>[4x]MNAAAVTPPPEKFNFAEHLLQTNRVRPDKTAFVDDISSLSFAQLEAQTRQLAAALRAIGVKREERVLLLMLDGTDWPVAFLGAIYAGIVPVAVNTLLTADDYAYMLEHSRAQAVLVSGALHPVLKAALTKSDHEVQRVIVSRPAAPLEPGEVDFAEFVGAHAPLEKPAATQADDPAFWLYSSGSTGRPKGVVHTHANPYWTSELYGRNTLHLREDDVCFSAAKLFFAYGLGNALTFPMTVGATTLLMGERPTPDAVFKRWLGGVGGVKPTVFYGAPTGYAGMLAAPNLPSRDQVALRLASSAGEALPAEIGQRFQRHFGLDIVDGIGSTEMLAAFLSNLPDRVRYGTTGWPVPGYQIELRGDGGG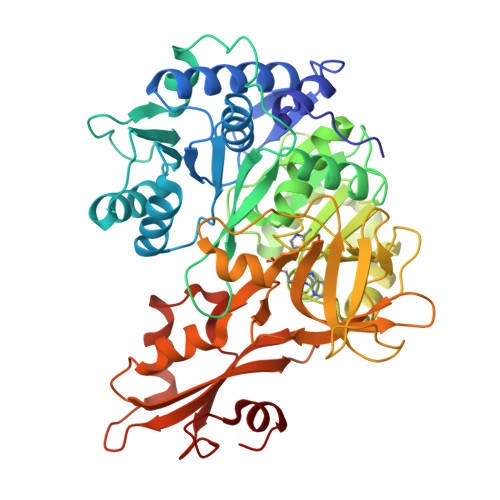PVADGEPGDLYIHGPSSATMYWGNRAKSRDTFQGGWTKSGDKYVRNDDGSYTYAGRTDDMLKVSGIYVSPFEIEATLVQHPGVLEAAVVGVADEHGLTKPKAYVVPRPGQTLSETELKTFIKDRLAPYKYPRSTVFVAELPKTATGKIQRFKLREGVLG>MSLKQKILIVEDSMTIRRMLIQAIAQQTGLEIDAFDTLEGARHCQGDEYVVALVDLTLPDAPSGEAVKVLLERGLPVVILTADISEDKREAWLEAGVLDYVMKDSRHSLQYAVGLVHRLYLNQQIEVLVVDDSRTSRHRTMAQLRKQLLQVHEASHAREALATLEQHPAIRLVLVDYYMPEIDGISL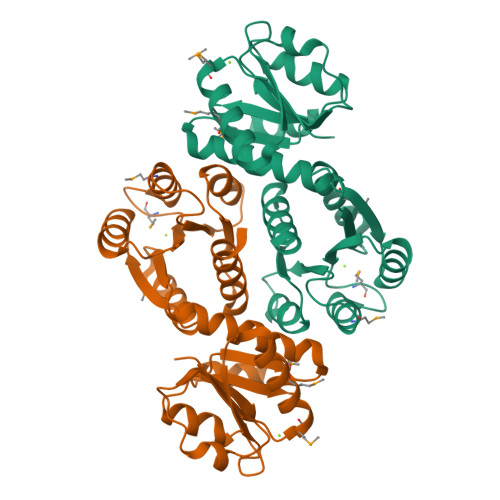VRMLRERYSKQQLAIIGISVSDKRGLSARYLKQGANDFLNQPFEPEELQCRVSHNLEALEQFNSEGHHHHHH[2x]>[2x]GPQDNPYERGPDPTEDSIEAIRGPFSVATERVSSFASGFGGGTIYYPRETDEGTFGAVAVAPGF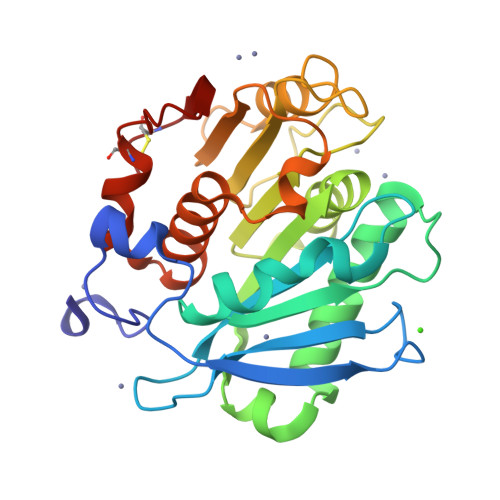TASQGSMSWYGERVASQGFIVFTIDTNTRLDQPGQRGRQLLAALDYLVERSDRKVRERLDPNRLAVMGHSMGGGGSLEATVMRPSLKASIPLTPWNLDKTWGQVQVPTFIIGAELDTIAPVSTHAKPFYESLPSSLPKAYMELDGATHFAPNIPNTTIAKYVISWLKRFVDEDTRYSQFLCPNPTDRAIEEYRSTCPY> MRIVVTGGAG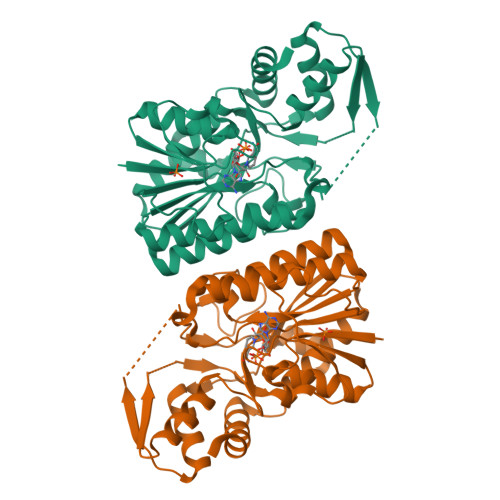FIGSHLVDKLVELGYEVVVVDNLSSGRREFVNPSAELHVRDLKDYSWGAGIKGDVVFHFAANPEVRLSTTEPIVHFNENVVATFNVLEWARQTGVRTVVFASSSTVYGDADVIPTPEEEPYKPISVYGAAKAAGEVMCATYARLFGVRCLAVRYANVVGPRLRHGVIYDFIMKLRRNPNVLEVLGDGTQRKSYLYVRDAVEATLAAWKKFEEMDAPFLALNVGNVDAVRVLDIAQIVAEVLGLRPEIRLVPSTPDGRGWPGDVKYMTLAVTKLMKLTGWRPTMTSAEAVKKTAEDLAKELWG> MKRQGKRPSKNLKARCSRKALHVNFKDMGWDDWIIAPLEYEAFHCEGLCEFPLRSHLEPTNHAVIQTLMNSMDPESTPPTCCVPTRLSPISILFIDSANNVVYKQYEDMVVESCGCR;> GSGAMA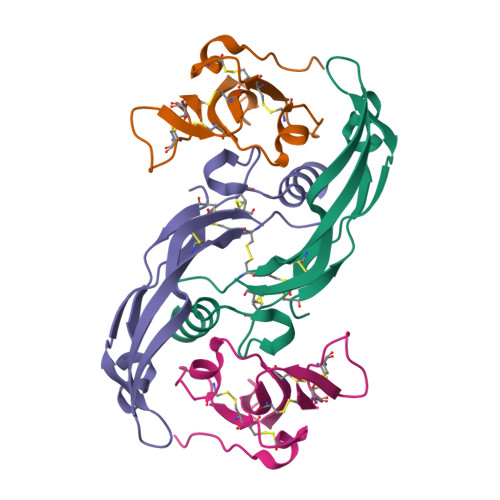KKEDGESTAPTPRPKILRCKCHHHCPEDSVNNICSTDGYCFTMIEEDDSGMPVVTSGCLGLEGSDFQCRDTPIPHQRRSIECCTERNECNKDLHPTLPPLKDRDFVDGPIHHK Porphyridium cruentum is a red marine microalga, reservoir of potentially high-added value molecules, such as carotenoids, sulfated exopolysaccharides (EPSs), B-phycoerythrin (PE), and lipids. Carotenoids are well-known antioxidants, also able to counteract many disorders, from type 2 diabetes, to degenerative diseases or cancer. PE, the main protein found inP. cruentum, has a good market value for different reasons: (i) in biomedical and molecular applications for its natural fluorescence; (ii) as a natural red-colored protein to be used as a dye for food and cosmetics, and (iii) in the pharmaceutical industry thanks to its antioxidant activity. The analyses revealed two major bands, whose molecular weights corresponded to α and β subunits (17 kDa) and γ subunit (30 kDa) of PE, in each lane.

To the best of our knowledge, this is the first time that PE was extracted and purified with such a purity grade by using only a single purification step. To determine the protein identity and purity, PE was crystallized, and its X-ray structure was determined at 1.60 Å resolution. The X-ray structure is constituted by 5990 atoms, including five phycoerythrobilin (PEB) chromophores for each αβ dimer, one methylated Asn in position β72 for each β subunit, two sulfate ions, and 324 water molecules and refines to R factor/Rfree values of 0.222/0.256. The structure confirms the formation of the (αβ)3 hexamer but does not allow to identify the exact location of the γ subunit. The α subunit contains 164 residues, the β subunit 177 residues. Each αβ dimer has five PEBs in position α82, α139, β61, β82, and β158. The first PEB, which adopts two alternate conformations in our structure, is covalently attached to the side chain of Cys82 of the α subunit by ring A. The second PEB is bound to Cys139 of the same subunit. The other three PEBs are found in the β subunit. They are bound to the side chains of Cys61, Cys82, and Cys158. The UV–vis absorption spectrum showed a peculiar shoulder at 498 nm, ascribed to the phycourobilin chromophore of the γ subunit.

>MKSVITTVVSAADAAGRFPSNSDLESIQGNIQRSAARLEAAEKLAGNHEAVVKEAGDACFAKYAYLKNPGEAGENQEKINKCYRDVDHYMRLVNYCLVVGGTGPLDEWGIAGAREVYRTLNLPTSAYVASIAYTRDRLCVPRDMSAQAGVEFSAYLDYLINALS[2x];>[2x]MLDAFSRVVVNSDAKAAYVGGSDLQALKSFIADGNKRLDAVNSIVSNASCMVSDAVSGMICENPGLISPGGNCYTNRRMAACLRDGEIILRYVSYALLAGDASVLEDRCLNGLKETYIALGVPTNSSIRAVSIMKAQAVAFITNTATERKMSFAAGDCTSLASEVASYFDRVGAAIS> GSMDYKDD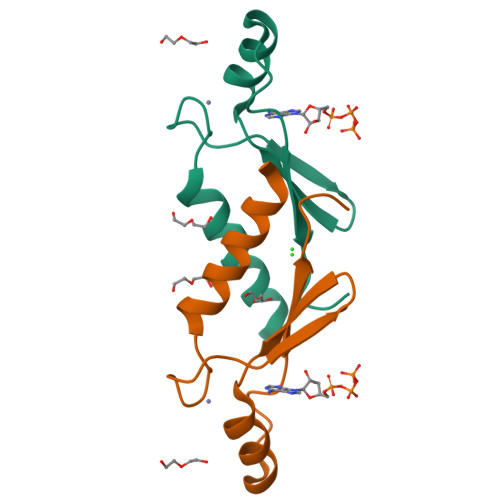DDKKTNWLKRIYRVRPCVKCKVAPRDWKVKNKHLRIFNMCKTCFNNSIDIGDDTYHGHVDWLMYADSKEISNT>[4x]MTSLVVPGLDTLRQWLDDLGMSFFECDNCQALHLPHMQNFDGVFDAKIDLIDNTILFSAMAEVRPSAVLPLAADLSAI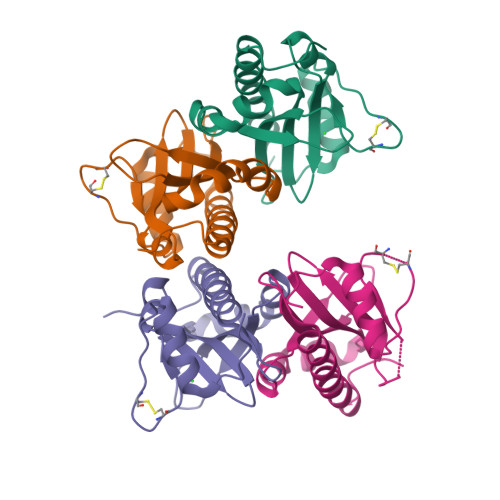NASSLTVKAFLDMQDDNLPKLVVCQSLSVMQGVTYEQFAWFVRQSEEQISMVILEANAHQLLLPTDDEGQNNVTENYFLH4-amino-N-(1,3-thiazol-2-yl)benzenesulfonamide | C9 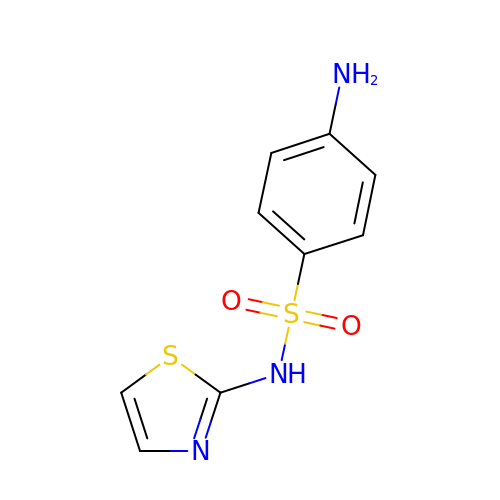H9 N3 O2 S2 | JNMRHUJNCSQMMB-UHFFFAOYSA-N> MSVNALYDYKFEPKDKVENFHGMQL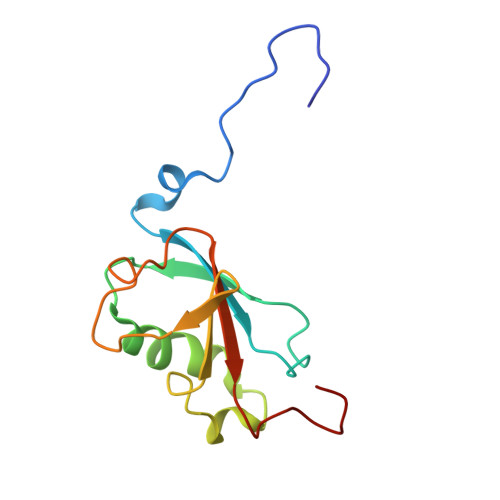LYVYWPDHLLFCAPFALLVQPGMTFSALVDEILKPATAAHPDSAKADFLNAEWLLNDEPFTPKADASLKEQGIDHKSMLTVTTPGLKGMANAGY>[4x]SRKTYTLTDYLKNTYRLKLYSLRWISDHEYLYKQENNILVFNAEYGNSSVFLENSTFDEFGHSINDYSISPDGQFILLEYNYVKQWRHSYTASYDIYDLNKRQLITEERIPNNTQWVT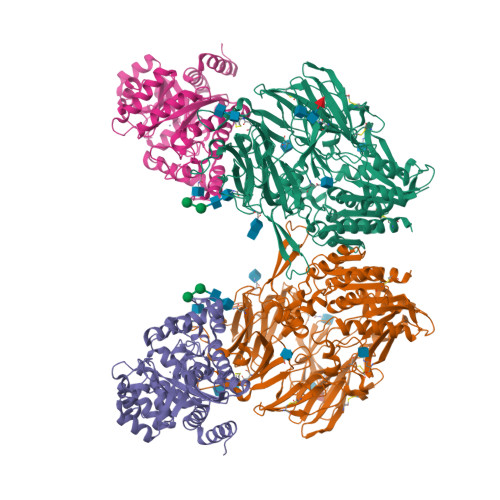WSPVGHKLAYVWNNDIYVKIEPNLPSYRITWTGKEDIIYNGITDWVYEEEVFSAYSALWWSPNGTFLAYAQFNDTEVPLIEYSFYSDESLQYPKTVRVPYPKAGAVNPTVKFFVVNTDSLSSVTNATSIQITAPASMLIGDHYLCDVTWATQERISLQWLRRIQNYSVMDICDYDESSGRWNCLVARQHIEMSTTGWVGRFRPSEPHFTLDGNSFYKIISNEEGYRHICYFQIDKKDCTFITKGTWEVIGIEALTSDYLYYISNEYKGMPGGRNLYKIQLSDYTKVTCLSCELNPERCQYYSVSFSKEAKYYQLRCSGPGLPLYTLHSSVNDKGLRVLEDNSALDKMLQNVQMPSKKLDFIILNETKFWYQMILPPHFDKSKKYPLLLDVYAGPCSQKADTVFRLNWATYLASTENIIVASFDGRGSGYQGDKIMHAINRRLGTFEVEDQIEAARQFSKMGFVDNKRIAIWGWSYGGYVTSMVLGSGSGVFKCGIAVAPVSRWEYYDSVYTERYMGLPTPEDNLDHYRNSTVMSRAENFKQVEYLLIHGTADDNVHFQQSAQISKALVDVGVDFQAMWYTDEDHGIASSTAHQHIYTHMSHFIKQCFSLP;>MAQTPAFDKPKVELHVHLDGAIKPETILYYGKRRGIALPADTPEELLNIIGMDKPLTLPDFLAKFDYYMPAIAGCRDAIKRIAYEFVEMKAKDGVVYVEVRYSPHLLANSKVEPIPWNQAEGDLTPDEVVSLVNQGLQEGERDFGVKVRSILCCMRHQPSWSSEVVELCKKYREQTVVAIDLAGDETIEGSSLFPGHVQAYAEAVKSGVHRTVHAGEVGSANVVKEAVDTLKTERLGHGYHTLEDTTLYNRLRQENMHFEICPWSSYLTGAWKPDTEHAVIRFKNDQVNYSLNTDDPLIFKSTLDTDYQMTKKDMGFTEEEFKRLNINAAKSSFLPEDEKKELLDLLYKAYRMPSPA[4x]>AAATTT[3x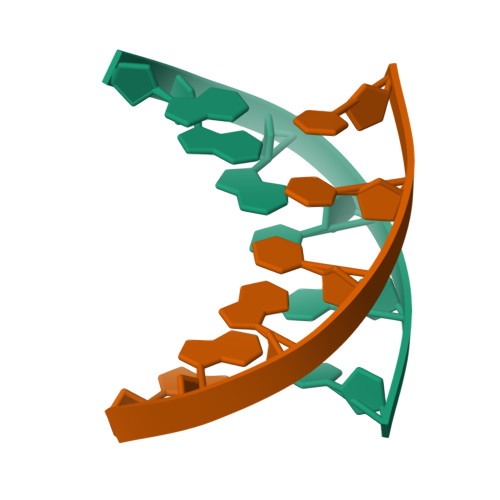]>[2x]ELTPDQQTLLHFIMDSYNKQRMPQEITNKILKEEFSAEENFLILTEMATNHVQVLVEFTKKLPGFQTLDHEDQIALLKGSAVEAMFLRSAEIFNKKLPSGHSDLLEERIR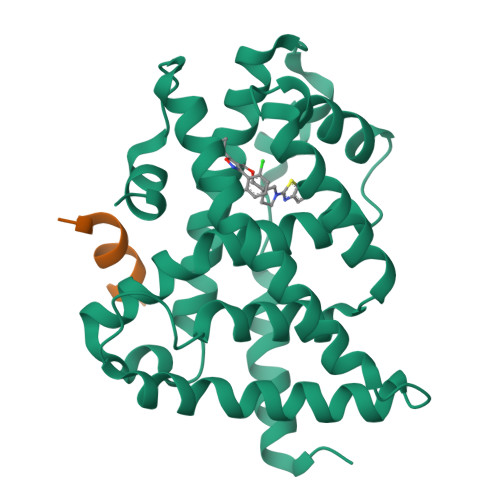NSGISDEYITPMFSFYKSIGELKMTQEEYALLTAIVILSPDRQYIKDREAVEKLQEPLLDVLQKLCKIHQPENPQHFAELLGRLTELRTFNHHHAEMLMSWRVNDHKFTPLLEEIWDV;>DHQLLRYLLDKD[2x]> GVPTYLLPGSGQFLTTDDHSSAPALPCFNPTPEMHIPGQVRNMLEVVQVESMMEINNTESAVGMERLKVDISALTDVDQLLFNIPLDIQLDGPLRNTLVGNISRYYTHWSGSLEMTFMFCGSFMAAGKLILCYTPPGGSCPTTRETAMLGTHIVW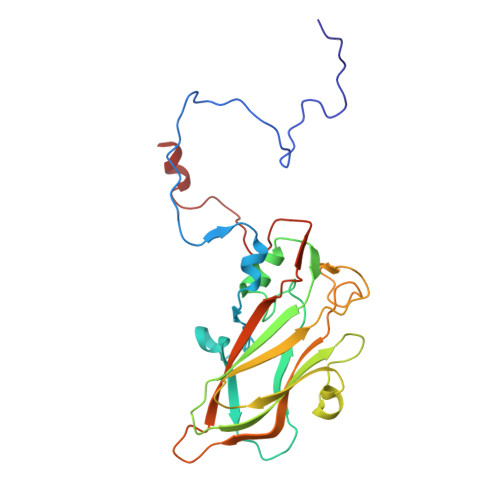DFGLQSSVTLIIPWISGSHYRMFNNDAKSTNANVGYVTCFMQTNLIVPSESSDTCSLIGFIAAKDDFSLRLMRDSPDIGQLDHLHAAEAAYQ>[2x]QCYHG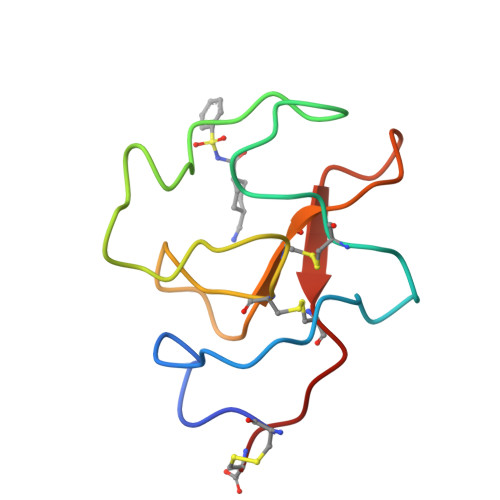NGQSYRGTFSTTVTGRTCQSWSSMTPHRHQRTPENYPNDGLTMNYCRNPDADTGPWCFTMDPSIRWEYCALTRC>MQRALTRASVSSPLATARVRSAQQLRFAHKELKFGVEGRAALLNGVETLAKAVATTLGPKGRNVLIESTFGSPKITKDGVTVAKAISLKDKFENLGAKLLAEVASKTNEVAGDGTTTATVLARAIFSEMVKNVAAGCNPMDLRRGIQAAVDAVVEYLQQNKRDITTSAEIAQVATISANGDQHIGKLIASAMEKVGKEGVITVKEGKTLQDELEVTEGMRFDRGFVSP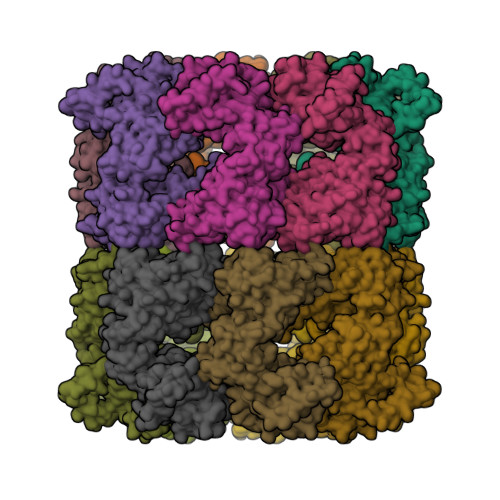YFITDAKAQKVEFEKPLILLSEQKISAATDIIPALEISHKMRRPLVIIAEDIDGEALAVCILNKLRGQLEVAAVKAPGFGDNRKSILGDIAVLTNGTVFTNELDVKLEKVTPDMLGSTGSITITKEDTIILNGDGSKDAIAQRCEQIRGAMNDPSTSEYEKEKLQERLAKLSGGVAVIKVGGSSEVEVGEKKDRFVDALNATRAAVEEGILPGGGTALIKASVNALNNLKPANFDQQLGVNIIKNAITRPARMIVENAGLEGSVVIGKISDEYAADFNKGFNSATGEYVDMIQAGILDPLKVVRTGLIDASGVASLLGTTEVAIVEAPEEKGPAGGMGGMGGMGGMM[14x]>[2x]MLWSSNDVTQQGSRPKTKLGGSMSIIATVKIGPDEISA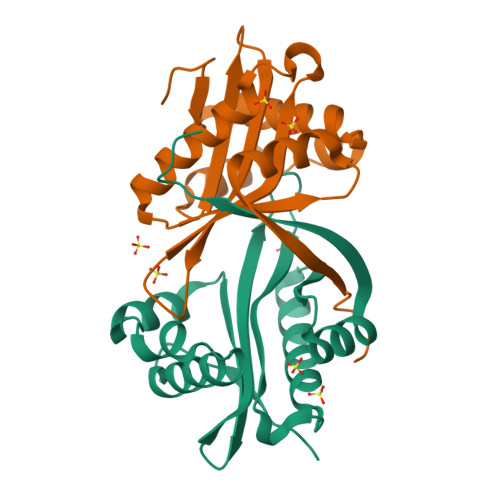MRAVLDLFGKEFEDIPTYSDRQPTNEYLANLLHSETFIALAAFDRGTAIGGLAAYVLPKFEQARSEIYIYDLAVASSHRRLGVATALISHLKRVAVELGAYVIYVQADYGDDPAVALYTKLGVREDVMHFDIDPRTATHHHHHH>[2x]MGSSHHHHHHSSGENLYFQGHM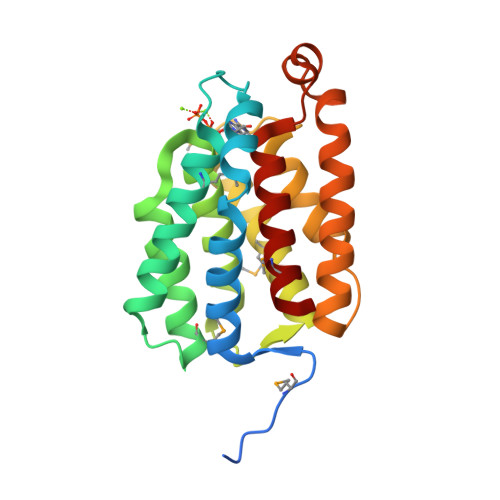AEAWGPEAVAEAFRYATRWFQVYVEELNALNVYPVPDGDTGTNMLHTLEAARRELDLADTSRMDQVARALAYGSLLGARGNSGVILSQILRGFAEALKGKRALDGSLLRRALRMGAESGYKAVMRPVEGTILTVARAAGEGARGEALEEVLETALEAAREALERTPELLPVLRQAGVVDAGGAGYVRLLEGMRGYAL>GAPIHDPDFIGGIGKELIVDNASDVTSFYPSAFQEHLNFIPAPTTGSGCTRIPSFDMSATHYCYTHNVILSGCRDHSHSHQYLALGVLRTTATGRIFFSTLRSISLDDTQNRKSCSVSATPLGCDMLCSKVTETEEEDYNSAVPTLMAHGRLGFDGQYHEKDLDVTTLFEDWVANYPGVGGGSFIDGRVWFSVYGGLKPNSPSDTVQEGKYVIYKRYNDTCPDEQDYQIRMAKSSYKPGRFGGKRIQQAILSIKVSTSLGEDPVL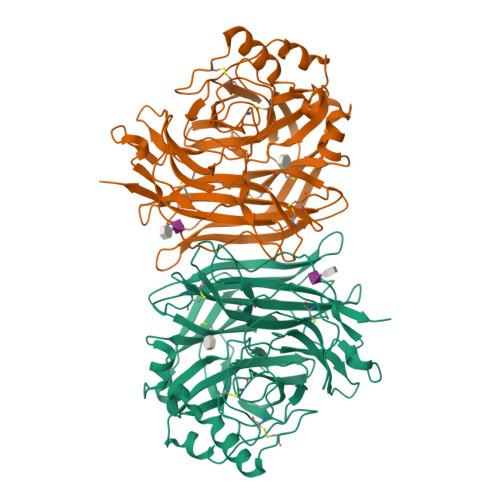TVPPNTVTLMGAEGRILTVGTSHFLYQRGSSYFSPALLYPMTVSNKTATLHSPYTFNAFTRPGSIPCQASARCPNSCVTGVYTDPYPLIFYRNHTLRGVFGTMLDSEQARLNPASAVFDSTSRSRITRVSSSSTKAAYTTSTCFKVVKTNKTYCLSIAEISNTLFGEFRIVPLLVEILKNDGVREARSG[3x]> KVFERCELARTLKRLG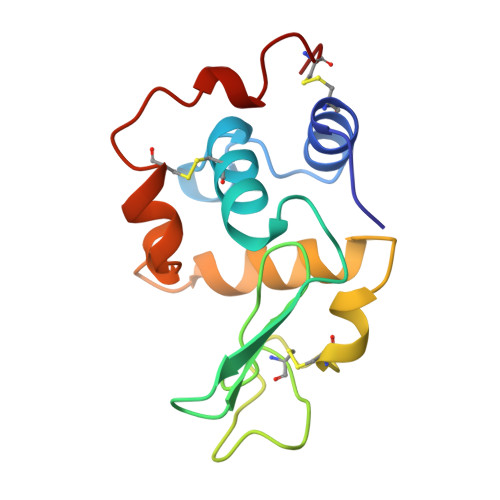MDGYRGISLANWMCLAKWESGYNTRATNYNAGDRSTDYGIFQINSRYWCNDGKTPGAVNAAHLSCSALLQDNIADAVAAAKRVVRDPQGIRAWAAWRNRCQNRDVRQYVQGCGV>[2x]HQKYNPFRFVELVLVVDKAMVTKNNGDLDKIKTRMYEIVNTVNEIYRYMYIHVALVGLEIWSNEDKITVKPEAGYTLNAFGEWRKTDLLTRKKH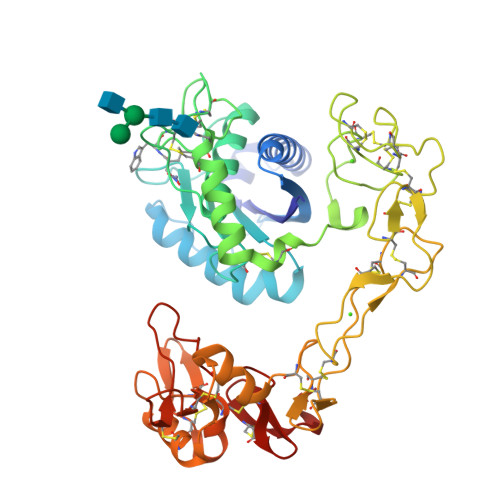DNAQLLTAIDLDRVIGLAYVGSMCHPKRSTGIIQDYSEINLVVAVIMAHEMGHNLGINHDSGYCSCGDYACIMRPEISPEPSTFFSNCSYFECWDFIMNHNPECILNEPLGTDIISPPVCGNELLEVGEECDCGTPENCQNECCDAATCKLKSGSQCGHGDCCEQCKFSKSGTECRASMSECDPAEHCTGQSSECPADVFHKNGQPCLDNYGYCYNGNCPIMYHQCYDLFGADVYEAEDSCFERNQKGNYYGYCRKENGNKIPCAPEDVKCGRLYCKDNSPGQNNPCKMFYSNEDEHKGMVLPGTKCADGKVCSNGHCVDVATAY>MALQLSREQGITLRGSAEIVAEFFSFGINSILYQRGIYPSETFTRVQKYGLTLLVTTDLELIKYLNNVVEQLKDWLYKCSVQKLVVVISNIESGEVLERWQFDIECDKTAKDDSAPREKSQKAIQDEIRSVIAQITATVTFLPLLEVSCS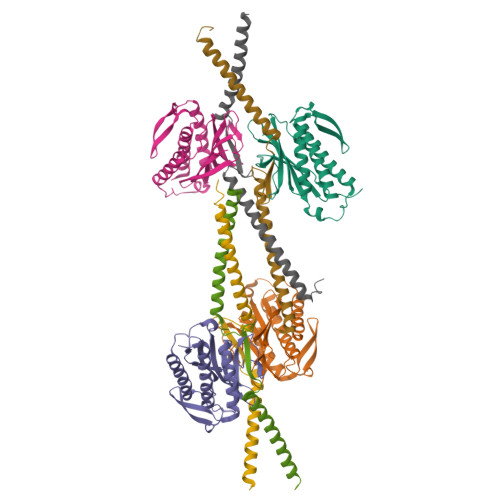FDLLIYTDKDLVVPEKWEESGPQFITNSEEVRLRSFTTTIHKVNSMVAYKIPVND[4x];>SSAEQSFLFSREEADTLRLKVEELEGERSRLEEEKRMLEAQLERRALQGDYDQSRTKVLHMSLNPTSVARQRLREDHSQLQAECERLRGLLRAMERGGTV[4x]> MVSSAQMGFNLQALLEQLSQDELSKFKYLITTFSLAHELQKIPHKEVDKADGKQLVEILTTHCDSYWVEMASLQVFEKMHRMDLSERAKDEVREAALKSFNKRKPLSLGITRKERPPLDVDEMLERFKTEAQAFTETKGNVICLGKEVFKGKKPDKDNRCRYILKTKFREMWKSWPGDSKEVQVMAERYKMLIPFSNPRVLPGPFSYTVVLYGPAGLGKTTLAQKLMLDWAEDNLIHKFKYAFYLSCRELSRLGPCSFAELVFRDWPELQDDIPHILAQARKILFVIDGFDELGAAPGALIEDICGDWEKKKPVPVLLGSLLNRVMLPKAALLVTTRPRALRDLRILAEEPIYIRVEGFLEEDRRAYFLRHFGDEDQAMRAFELMRSNAALFQLGSAPAVCWIVCTTLKLQMEKGEDPVPTCLTRTGLFLRFLCSRFPQGAQLRGALRTLSLLAAQGLWAQTSVLHREDLERLGVQESDLRLFLDGDILRQDRVSKGCYSFIHLSFQQFLTALFYTLEKEEEEDRDGHTWDIGDVQKLLSGVERLRNPDLIQAGYYSFGLANEKRAKELEATFGCRMSPDIKQELLRCDISCKGGHSTVTDLQELLGCLYESQEEELVKEVMAQFKEISLHLNAVDVVPSSFCVKHCRNLQKMSLQVIKENLPENVTASESDAEVERSQDDQHMLPFWTDLCSIFGSNKDLMGLAINDSFLSASLVRILCEQIASDTCHLQRVVFKNISPADAHRNLCLALRGHKTVTYLTLQGNDQDDMFPALCEVLRHPECNLRYLGLVSCSATTQQWADLSLALEVNQSLTCVNLSDNELLDEGAKLLYTTLRHPKCFLQRLSLENCHLTEANCKDLAAVLVVSRELTHLCLAKNPIGNTGVKFLCEGLRYPECKLQTLVLWNCDITSDGCCDLTKLLQEKSSLLCLDLGLNHIGVKGMKFLCEALRKPLCNLRCLWLWGCSIPPFSCEDLCSALSCNQSLVTLDLGQNPLGSSGVKMLFETLTCSSGTLRTLRLKIDDFNDELNKLLEEIEEKNPQLIIDTEKHHPWAERPSSHDFMI;> MVDDAGAAESQRGKQTPAHSLEQLRRLPLPPPQIRIRPWWFPVQELRDPLVFYLEAWLADELFGPDRAIIPEMEWTSQALLTVDIVDSGNLVEITVFGRPRVQNRVKSMLLCLAWFHREHRARAEKMKHLEKNLKAHASDPHSPQDPVA;> MTSRDQPRPKGPPKSTSPCPGISNSESSPTLNYQGILNRLKQFPRFSPHFAAELESIYYSLHKIQQDVAEHHKQIGNVLQIVESCSQLQGFQSEEVSPAEPASPGTPQQVKDKTLQESSFEDIMATRSSDWLRRPLGEDNQPETQLFWDKEPWFWHDTLTEQLWRIFAGVHDEKAKPRDRQQAPGLGQESKAPGSCDPGTDPCPEDASTPRPPEASSSPPEGSQDRNTSWGVVQEPPGRASRFLQSISWDPEDFEDAWKRPDALPGQSKRLAVPCKLEKMRILAHGELVLATAISSFTRHVFTCGRRGIKVWSLTGQVAEDRFPESHLPIQTPGAFLRTCLLSSNSRSLLTGGYNLASVSVWDLAAPSLHVKEQLPCAGLNCQALDANLDANLAFASFTSGVVRIWDLRDQSVVRDLKGYPDGVKSIVVKGYNIWTGGPDACLRCWDQRTIMKPLEYQFKSQIMSLSHSPQEDWVLLGMANGQQWLQSTSGSQRHMVGQKDSVILSVKFSPFGQWWASVGMDDFLGVYSMPAGTKVFEVPEMSPVTCCDVSSNNRLVVTGSGEHASVYQITY;> MKVAGGLELGAAALLSASPRALVTLSTGPTCSILPKNPLFPQNLSSQPCIKMEGDKSLTFSSYGLQWCLYELDKEEFQTFKELLKKKSSESTTCSIPQFEIENANVECLALLLHEYYGASLAWATSISIFENMNLRTLSEKARDDMKRHSPEDPEATMTDQGPSKEKVPGISQAVQQDSATAAETKEQEISQAMEQEGATAAETEEQEISQAMEQEGATAAETEEQGHGGDTWDYKSHVMTKFAEEEDVRRSFENTAADWPEMQTLAGAFDSDRWGFRPRTVVLHGKSGIGKSALARRIVLCWAQGGLYQGMFSYVFFLPVREMQRKKESSVTEFISREWPDSQAPVTEIMSRPERLLFIIDGFDDLGSVLNNDTKLCKDWAEKQPPFTLIRSLLRKVLLPESFLIVTVRDVGTEKLKSEVVSPRYLLVRGISGEQRIHLLLERGIGEHQKTQGLRAIMNNRELLDQCQVPAVGSLICVALQLQDVVGESVAPFNQTLTGLHAAFVFHQLTPRGVVRRCLNLEERVVLKRFCRMAVEGVWNRKSVFDGDDLMVQGLGESELRALFHMNILLPDSHCEEYYTFFHLSLQDFCAALYYVLEGLEIEPALCPLYVEKTKRSMELKQAGFHIHSLWMKRFLFGLVSEDVRRPLEVLLGCPVPLGVKQKLLHWVSLLGQQPNATTPGDTLDAFHCLFETQDKEFVRLALNSFQEV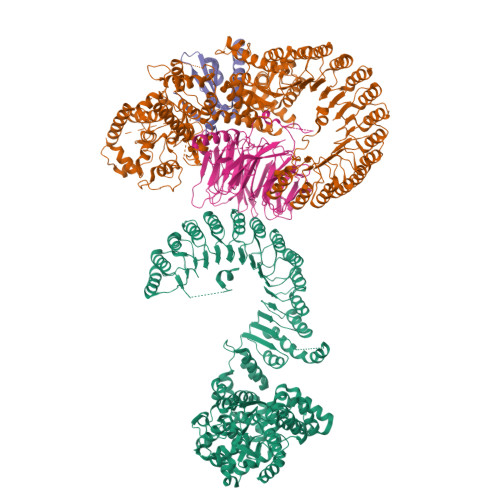WLPINQNLDLIASSFCLQHCPYLRKIRVDVKGIFPRDESAEACPVVPLWMRDKTLIEEQWEDFCSMLGTHPHLRQLDLGSSILTERAMKTLCAKLRHPTCKIQTLMFRNAQITPGVQHLWRIVMANRNLRSLNLGGTHLKEEDVRMACEALKHPKCLLESLRLDCCGLTHACYLKISQILTTSPSLKSLSLAGNKVTDQGVMPLSDALRVSQCALQKLILEDCGITATGCQSLASALVSNRSLTHLCLSNNSLGNEGVNLLCRSMRLPHCSLQRLMLNQCHLDTAGCGFLALALMGNSWLTHLSLSMNPVEDNGVKLLCEVMREPSCHLQDLELVKCHLTAACCESLSCVISRSRHLKSLDLTDNALGDGGVAALCEGLKQKNSVLARLGLKACGLTSDCCEALSLALSCNRHLTSLNLVQNNFSPKGMMKLCSAFACPTSNLQIIGLWKWQYPVQIRKLLEEVQLLKPRVVIDGSWHSFDEDDRYWWKN> MANMKNSNDRIILFRKAGEKVDATKMLFLTEYGLSHEADTDTEDTMDGSYNTGGSVESTMSGTAKMFYGDDFADEIEDAVVDRVLYEAWEVES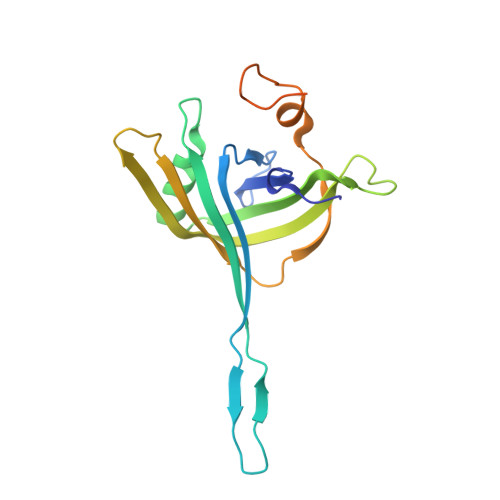RIPGKNGDSAKFKAKYFQGFHNKFELKAEANGIDEYEYEYGVNGRFQRGFATLPEAVTKKLKATGYRFHDTTKEDALTSEDLTAIPQPKVDSSTVTPGEV>GIDP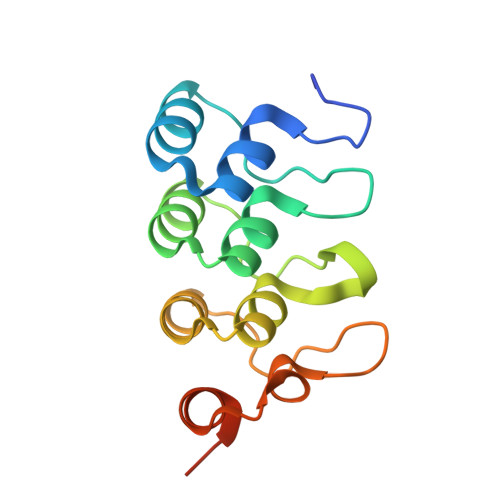FTNHRGETLLHIASIKGDIPSVEYLLQNGSDPNVKDHAGWTPLHEACNHGHLKVVELLLQHKALVNTTGYQNDSPLHDAAKNGHVDIVKLLLSYGASRNAVNIFGLRPVDYTDDESMKSLLLLPEKNESSSAS[2x]> MASHKLLVTPPKALLKPLSIPNQLLLGPGPSNLPPRIMAAGGLQMIGSMSKDMYQIMDEIKEGIQYVFQTRNPLTLVISGSGHCALEAALVNVLEPGDSFLVGANGIWGQRAVDIGERIGARVHPMTKDPGGHYTLQEVEEGLAQHKPVLLFLTHGESSTGVLQPLDGFGELCHRYKCLLLVNSVASLGGTPLYMDRQGIDILYSGSQKALNAPPGTSLISFSDKAKKKMYSRKTKPFSFYLDIKWLANFWGCDDQPRMYHHTIPVISLYSLRESLALIAEQGLENSWRQHREAAAYLHGRLQALGLQLFVKDPALRLPTVTTVAVPAGYDWRDIVSYVIDHFDIEIMGGLGPSTGKVLRIGLLGC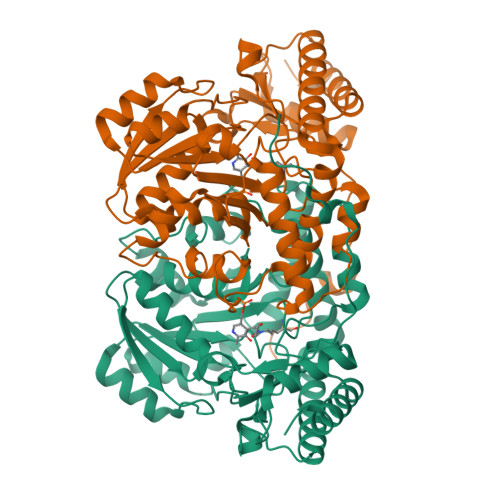NATRENVDRVTEALRAALQHCPKKKL> SADAQSFLNRVCGVSAARLTPCGTGTSTDVVYRAFDIYNDKVAGFAKFLKTNCCRFQEKDEDDNLIDSYFVVKRHTFSNYQHEETIYNLLKDCPAVAKHDFFKFRIDGDMVPHISRQRLTKYTMADLVYALRHFDEGNCDTLKEILVTYNCCDDDYFNKKDWYDFVENPDILRVYANLGERVRQALLKTVQFCDAMRNAGIVGVLTLD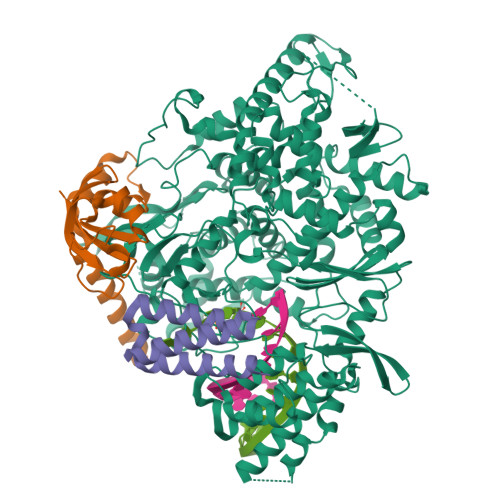NQDLNGNWYDFGDFIQTTPGSGVPVVDSYYSLLMPILTLTRALTAESHVDTDLTKPYIKWDLLKYDFTEERLKLFDRYFKYWDQTYHPNCVNCLDDRCILHCANFNVLFSTVFPPTSFGPLVRKIFVDGVPFVVSTGYHFRELGVVHNQDVNLHSSRLSFKELLVYAADPAMHAASGNLLLDKRTTCFSVAALTNNVAFQTVKPGNFNKDFYDFAVSKGFFKEGSSVELKHFFFAQDGNAAISDYDYYRYNLPTMCDIRQLLFVVEVVDKYFDCYDGGCINANQVIVNNLDKSAGFPFNKWGKARLYYDSMSYEDQDALFAYTKRNVIPTITQMNLKYAISAKNRARTVAGVSICSTMTNRQFHQKLLKSIAATRGATVVIGTSKFYGGWHNMLKTVYSDVENPHLMGWDYPKCDRAMPNMLRIMASLVLARKHTTCCSLSHRFYRLANECAQVLSEMVMCGGSLYVKPGGTSSGDATTAYANSVFNICQAVTANVNALLSTDGNKIADKYVRNLQHRLYECLYRNRDVDTDFVNEFYAYLRKHFSMMILSDDAVVCFNSTYASQGLVASIKNFKSVLYYQNNVFMSEAKCWTETDLTKGPHEFCSQHTMLVKQGDDYVYLPYPDPSRILGAGCFVDDIVKTDGTLMIERFVSLAIDAYPLTKHPNQEYADVFHLYLQYIRKLHDELTGHMLDMYSVMLTNDNTSRYWEPEFYEAMYTPHTVLQ;> MGSSHHHHHHENLYFQSNAAIASEFSSLPSYAAFATAQEAYEQAVANGDSEVVLKKLKKSLNVAKSEFDRDAAMQRKLEKMADQAMTQMYKQARSEDKRAKVTSAMQTMLFTMLRKLDNDALNNIINNARDGCVPLNIIPLTTAAKLMVVIPDYNTYKNTCDGTTFTYASALWEIQQVVDADSKIVQLSEISMDNSPNLAWPLIVTALRANSAVKLQ;> SNASKMSDVKCTSVVLLSVLQQLRVESSSKLWAQCVQLHNDILLAKDTTEAFEKMVSLLSVLLSMQGAVDINKLCEEMLDNRAT> MTMRYQEPARIPNAEI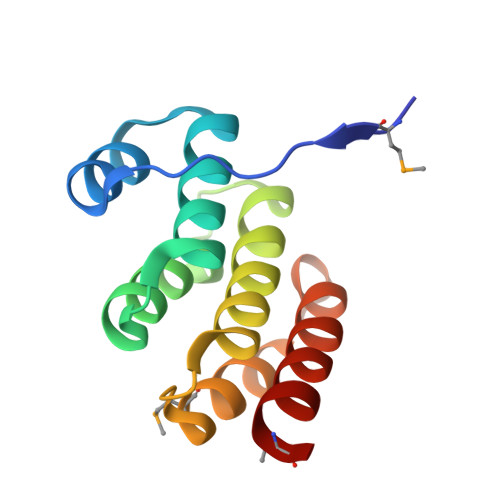DHVLASGNPEAIADACLSIAYYEDDWEWAFKRLKSVAFDLNRPDSLRSLAVTCVGHLARRIHDLDVAMAEEFLLSLGGDQAVASAASDALDDLRIFRMSD>MVNPRGLKPRVLWQMDVTHVSEFGKLKYVHVTVDTYSHFTFATARTGEATKDVLQHLAQSFAYMGIPQKIKTDNAPAYVSRSIQEFLARWKISHVTGIPYNPQGQAIVERTHQNIKAQLNKLQKAGK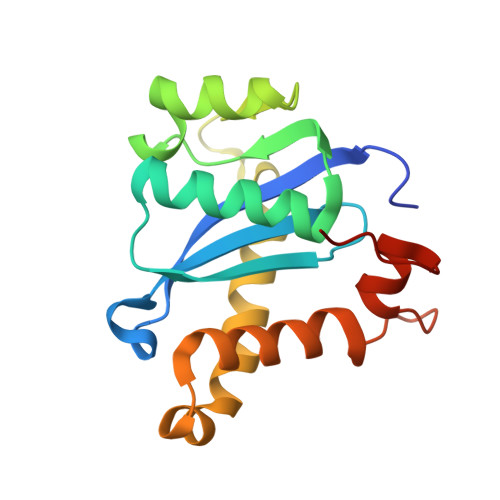YYTPHHLLAHALFVLNHVNMDNQGHTAAERHWGPISLEVLFQ[4x]> MGRMLTIRVFKYDPQSAV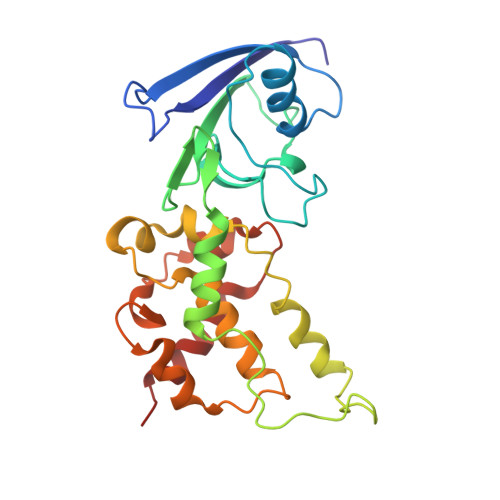SKPHFQEYKIEEAPSMTIFIVLNMIRETYDPDLNFDFVCRAGICGSCGMMINGRPSLACRTLTKDFEDGVITLLPLPAFKLIKDLSVDTGNWFNGMSQRVESWIHAQKEHDISKLEERIEPEVAQEVFELDRCIECGCCIAACGTKIMREDFVGAAGLNRVVRFMIDPHDERTDEDYYELIGDDDGVFGCMTLLACHDVCPKNLPLQSKIAYLRRKMVSVN> CASAPDNEPQGRSDPLEGFNRTMFDFNYNVLD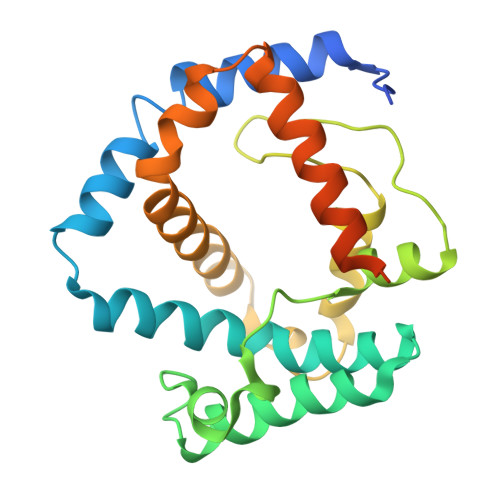PYILRPVAVAWRDYVPMPARNGISNFTSNLEEPASMVNAFLKGDPYRGMIHFNRFFLNTLLGMGGLIDVAGMANPKLAREEPNRFGSTLGHYDVGYGPYVMLPGYGSFTLRDEGGDFADTLYPMLSYLTFWMSAGKWVVEGIETRAQLLDSDGLLRNSSDPYIMVREAYFQRHDFIANGGSLKPEENPNAKAIQGELDEIDSQ>[2x]MIDVRKYIDNAALKPHLSEKEIEEFVLKSEELGIYAVCVNPYHVKLASSIAKKVKVCCVIGFPLGLNKTSVKVKEAVEAVRDG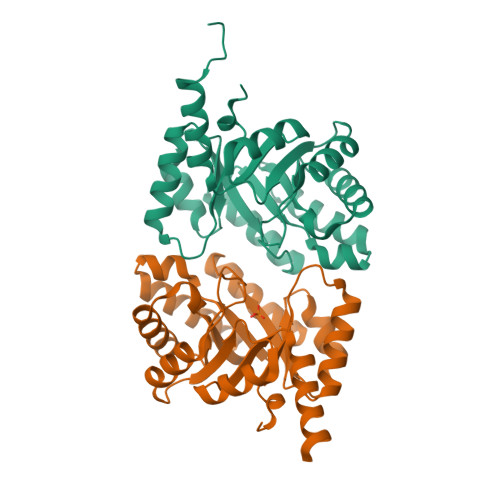AQELDIVWNLSAFKSEKYDFVVEELKEIFRETPSAVHKVIVETPYLNEEEIKKAVEICIEAGADFIKTSTGFAPRGTTLEEVRLIKSSAKGRIKVKASGGIRDLETAISMIEAGADRIGTSSGISIAEEFLKRHLILEHHHH>[2x]MAPALNANPTTKRDELSAPSASHKLGMSSMASRAAGGGLKLTGLPDLSDSTGTLSDIFGTPQMREIWSDQNRVACYLEIEAALAIVQADLGIIPKNAAHEIVEHCRVQEIDWALYKQK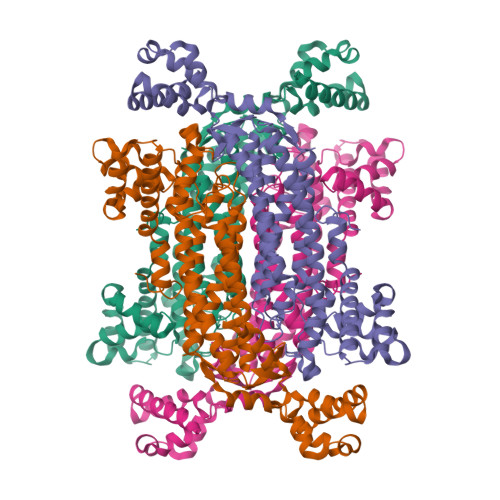TELIGYPVLGIVQQLVANCKDGLGEYCHWGATTQDITDTATVMQIRQSLTLVKQRLDSIVSSLEHLAEQHRNVPMAARSNLKQAVPITFGFKMARFLATFRRHQQRLVELEKRVYTLEFGGAAGNLSSLGDQGIATHDALAKMLDLAPAEIAWHTEHDRFAEVGTFLGLLTGTLAKLATDIKLMSQTEVGEVGEPFISNRGASSTMPQKNNPISCVYIHACAANVRQGAAALLDAMQSDHERGTGPWEIIWVQLPLMMNWTSAALNNADFVLRGLQVFPDAMQHNLDLSKGLIVSEAVMMGLGNTLGRQYAHDAVYECCRTAFVQDRPLLDVLLENHEIASKLDRTELEKLCDPANYLGQCSQWIDRVLSPPSSA> MGSNQSSSTSTKKLKAGNFDVAYQNPDKAIKGGNLKVAYQSDSPMKAQWLSGLSNDATFATMSGPGGGQDGLFFTDSGFKFIKGGAADVALDKESKTATITLRKDLKWSDGSEVTAKDYEFTYETIANPAYGSDRWTDSLANIVGLSDYHTGKAKTISGITFPDGENGKVIKVQFKE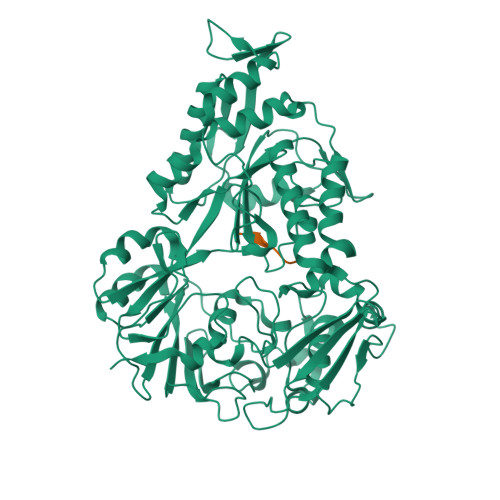MKPGMTQSGNGYFLETVAPYQYLKDVAPKDLASSPKTTTKPLVTGPFKPENVVAGESIKYVPNPYYWGEKPKLNSITYEVVSTAKSVAALSSSKYDIINGMVSSQYKQVKNLKGYKVLGQQAMYISLMYYNLGHYDAKNSINVQDRKTPLQDQNVRQAIGYARNVAEVDNKFSNGLSTPANSLIPPIFKQFTSSSVKGYEKQDLDKANKLLDEDGWKLNKSTGYREKDGKELSLVYAARVGDANAETIAQNYIQQWKKIGVKVSLYNGKLMEFNSWVDHMTTPPGANDWDITDGSWSLASEPSQQDLFSAAAPYNFGHFNDSEITKDLNDIDSAKSENPTYRKAAFVKYQEDMNKKAYVIPTNFMLNYTPVNKRVVGMTLDYGAMNTWSEIGVSSAKLATKGSIEGRHHHHHH;> AAAAAA> MKTPTIPTLLGPDGMTSLREYAGYHGGGSGFGGQLRSWNPPSESVDAAL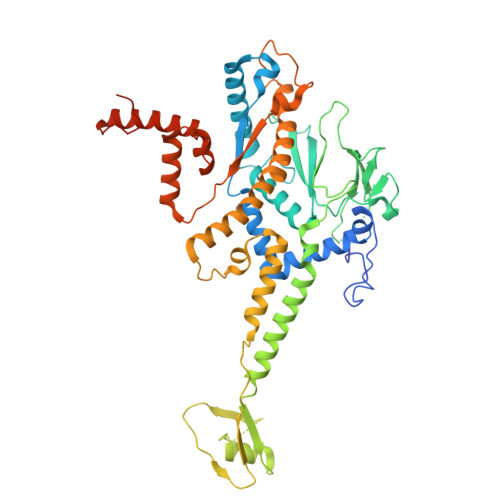LPNFTRGNARADDLVRNNGYAANAIQLHQDHIVGSFFRLSHRPSWRYLGIGEEEARAFSREVEAAWKEFAEDDCCCIDVERKRTFTMMIREGVAMHAFNGELFVQATWDTSSSRLFRTQFRMVSPKRISNPNNTGDSRNCRAGVQINDSGAALGYYVSEDGYPGWMPQKWTWIPRELPGGRASFIHVFEPVEDGQTRGANVFYSVMEQMKMLDTLQNTQLQSAIVKAMYAATIESELDTQSAMDFILGANSQEQRERLTGWIGEIAAYYAAAPVRLGGAKVPHLMPGDSLNLQTAQDTDNGYSVFEQSLLRYIAAGLGVSYEQLSRNYAQMSYSTARASANESWAYFMGRRKFVASRQASQMFLCWLEEAIVRRVVTLPSKARFSFQEARSAWGNCDWIGSGRMAIDGLKEVQEAVMLIEAGLSTYEKECAKRGDDYQEIFAQQVRETMERRAAGLKPPAWAAAAFESGLRQSTEEEKSDSRAA> MDETGKEL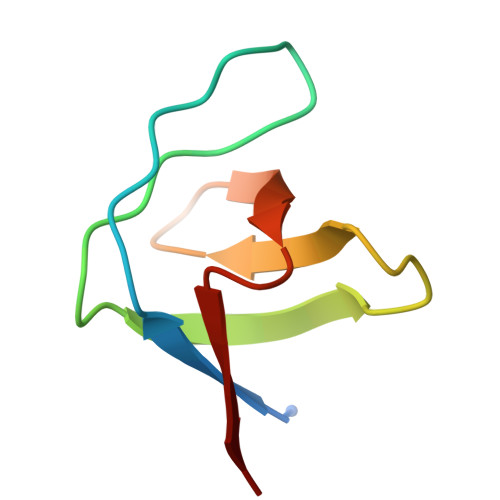VLALYDYQEKSPREVTMKKGDILTLLNSTNKDWWKVEVNDRQGFVPASYVKKLD>MSHSKQALADTMKMTWLMEGSVNGHAFTIEGEGTGKPYEGKQSGTFRVTKGGPLPFAFDIVAPTLKYGFKCFMKYPADIPDYFKLAFPEGLTYDRKIAFEDGGCATATVEMSLKGNTLVHKTNFQGGNFPIDGPVMQKRTLGWEPTSEKMTPCDGIIKGDTIMYLMVEGGKTLKCRYENNYRANKPVLMPPSHFVDLRLTRTNLDKEGLAFKLEEYAVARVLEV[4x]

Anthozoan chromoproteins are highly pigmented, diversely coloured and readily produced in recombinant expression systems. Here, high-resolution X-ray crystal structures of four open-source chromoproteins, gfasPurple, amilCP, spisPink and eforRed, are presented. Like GFP, chromoprotein monomers have a β-barrel structure that contains a chromophore, which is autocatalytically constructed from adjacent X–tyrosine–glycine residues encoded within the protein sequence itself.

Like other characterized chromoproteins, gfasPurple, amilCP and eforRed contain an sp 2-hybridized N-acylimine in the peptide bond preceding the chromophore, while spisPink is unusual and demonstrates a true sp 3-hybridized trans-peptide bond at this position. We believe that this is the first observed instance of a chromoprotein chromophore without N-acylimine formation. The closest structurally characterized protein to spisPink is the blue fluorescent protein amFP486 (53% sequence identity), which has the same KYG chromophore with sp 3 hybridization at this position. Of the four structures described in this work, the overall chromophore-binding site in spisPink is the most divergent from the others. The most striking difference is that Ser65 in gfasPurple, amilCP and eforRed, which forms a trans-peptide bond with N3 of the imidazolinone ring, is replaced by Phe69, adding considerable steric bulk in this region. The increased steric interactions displace the imidazolinone ring in spisPink relative to the same position in other chromoproteins, promoting the unusual twist in the tyrosyl moiety for its accommodation in the consequently smaller cavity.>MAHHHHHHVGTFENITAAPADPILGLADLFRADERPGKINLGIGAYIDETGKFPVLTSVKKAEQYLLENETTKSYLGIDGIPEFGRCTQELLFGKGSALINDKRARTAQTPGGTGALRVAADFLAKNTSVKRVWVSNPSWPNHKSVFNSAGLEVREYAYYDAENHTLDFDALINSLNEAQAGDVVLFHGCCHNPTGIDPTLEQWQTLAQLSVEKGWLPLFDFAYQGFARGLEEDAEGLRAFAAMHKELIVASSYSKNFGLYNERVGACTLVAADSETVDRAFSQMKAAIRANYSNPPAHGASVVATILSNDALRAIWEQELTDMRQRIQ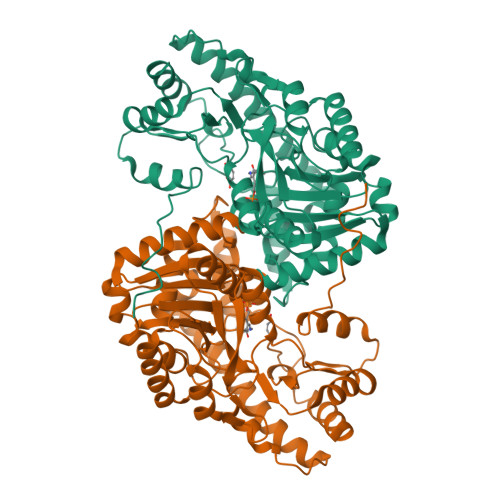RMRQLFVNTLQEKGANRDFSFIIKQNGMFSFSGLTKEQVLRLREEFGVYAVASGRVNVAGMTPDNMAPLCEAIVAVL[2x]> CAGCTGACCTGACTCAC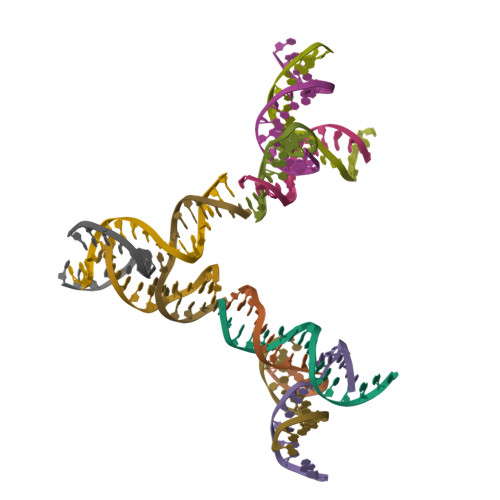A;> CGATGGACAGGGG;> TGTGAGTCACCATCG;> TGCTCCTGTGGTCAGC>[2x]MEFGSFLVSLGTSFVIFVILMLLFTWLSRKSGNAPIYYPNRILKGLEPWEGTSLTRNPFAWMREALTSSEQDVVNLSGVDTAVHFVFLSTVLGIFACSSLLLLPTLLPLAATDNNIKNTKNATDTTSKGTFSQLDNLSMANITKKSSRLWAFLGAVYWISLVTYFFLWKAYKHVSSLRAQALMSADVKPEQFAILVRDMPAPPDGQTQKEFIDSYFREIYPETFYRSLVATENSKVNKIWEKLEGYKKKLARAEAILAATNNRPTNKTGFCGLVGKQVDSIEYYTELINESVAKLETEQKAVLAEKQQTAAVVFFTTRVAAASAAQSLHCQMVDKWTVTEAPEPRQLLWQNLNIKLFSRIIRQYFIYFFVAVTIL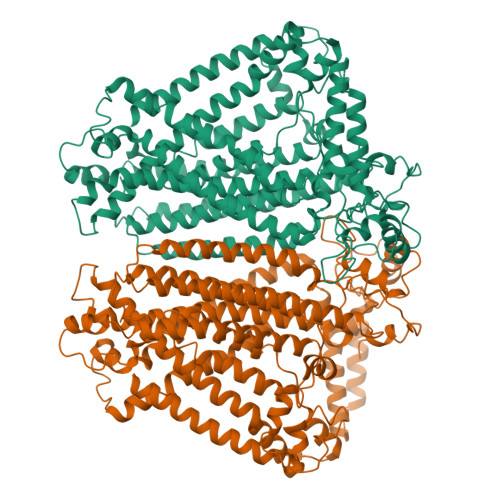FYMIPIAFVSAITTLKNLQRIIPFIKPVVEITAIRTVLESFLPQIALIVFLAMLPKLLLFLSKAEGIPSQSHAIRAASGKYFYFSVFNVFIGVTLAGTLFNTVKDIAKNPKLDMIINLLATSLPKSATFFLTYVALKFFIGYGLELSRIIPLIIFHLKKKYLCKTEAEVKEAWYPGDLSYATRVPGDMLILTITFCYSVIAPLILIFGITYFGLGWLVLRNQALKVYVPSYESYGRMWPHIHQRILAALFLFQVVMFGYLGAKTFFYTALVIPLIITSLIFGYVCRQKFYGGFEHTALEVACRELKQSPDLEEIFRAYIPHSLSSHKPEEHEFKGAMSRYQDFNAIAGV EFhd2/Swiprosin-1 (EFhd2) is a cytoskeletal Ca2+-binding protein identified in human immune, brain and mast cells. EFhd2 and EFhd1 consist of a disordered N-terminal region followed by two EF-hands and a coiled-coil domain at the C-terminus. We also reported previously that the EF-hands of EFhd2 are involved directly in F-actin bundling in a Ca2+-dependent manner and the coiled-coil domain is essential to the F-actin bundling activity by homodimerisation. Based on the experimental results, we propose that the F-actin bundling activity of EFhd2 depends on structural rigidity conferred by binding of two Ca2+ ions to the EF-hand domains.

We failed to determine the structure of the apo form of EFhd2 owing to structural instability during protein purification; however, we could determine the crystal structures of CDEFhd2 mutants defective for one Ca2+-binding site (E116A for EF1, CDEFhd2EF1; E152A for EF2, CDEFhd2EF2). The overall structures of these two mutants in the presence of Ca2+ are similar to that of Ca2+-bound CDEFhd2 (CDEFhd2EF1, root mean square deviation (RMSD) = 0.34 Å for 102 Cα atoms; CDEFhd2EF2, RMSD = 0.61 Å for 105 Cα atoms), which implies a single Ca2+-loaded EF-hand is sufficient to maintain a stable fold. Although the crystal structures of EF-hand mutants (CDEFhd2EF1 and CDEFhd2EF2) are similar to Ca2+-bound CDEFhd2, we observed structural flexibility in the Ca2+-binding loop of EF1 and the C-terminal linker. Furthermore, comparison of the crystallographic B-factors between Ca2+-bound and EF-hand mutant structures showed that the largest changes in B-factor values were for CDEFhd2EF1 (35.6 Å2), CDEFhd2 (20.4 Å2) and CDEFhd2EF2 (21.5 Å2). To evaluate the effect of Ca2+ on structural dynamics of EFhd2 at the atomic level, we performed ensemble refinement for CDEFhd2, CDEFhd2EF1 and CDEFhd2EF2 using Phenix.ensemble refinement. As expected, Ca2+-bound CDEFhd2 displayed a rigid conformation and CDEFhd2EF1 showed the largest degrees of mobility, indicating that Ca2+ depletion of EF1 has a larger impact on conformational dynamics. In addition, CDEFhd2EF2 also showed a moderate degree of mobility. Interestingly, the C-terminal linker (residues, 176–184) followed by the LM-helix also showed significant RMSF increases in CDEFhd2EF1 and CDEFhd2EF2. Consistent with a previous study showing that thermostability of EFhd2 was restored by Ca2+ at a high temperature, the half aggregation temperature for both EF-hand mutants that bind only one Ca2+ is significantly lower (CDEFhd2EF1: 62.32 ± 0.14 °C, CDEFhd2EF2: 57.90 ± 0.60 °C) than the two Ca2+-bound EFhd2 (CDEFhd2: 84.89 ± 0.01 °C) and is consistent with ref. Even depletion of one Ca2+ site in a two Ca2+-binding protein showed a dramatic reduction in F-actin bundling activity to a level that is similar to that of previously reported data for a two Ca2+-depleted state26.

> GAMGSGEPQSPSRRVFNPYTEFKEFSRKQIKDMEKMFKQYDAGRDGFIDLMALKLMMEKLGAPQTHLGLKNMIKEVDEDFDSKLSFREFLLIFRKAAAGELQEDSGLCVLARLSEIDVSS>[2x]GPNCAPGQKVKLFRASEPILSVLMWGVNHTINELSNVPVPVMLMPDD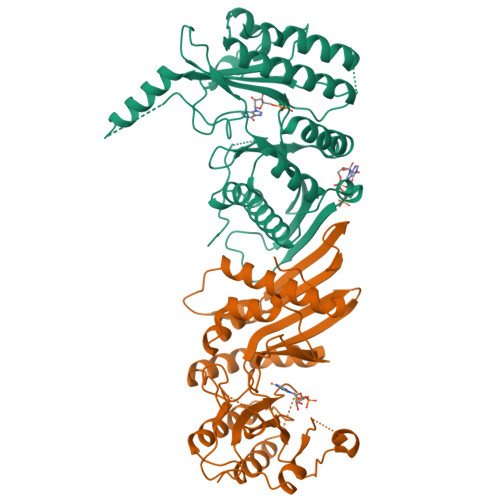FKAYSKIKVDNHLFNKENLPSRFKFKEYCPMVFRNLRERFGIDDQDYQNSVTRSAPINSDSQGRCGTRFLTTYDRRFVIKTVSSEDVAEMHNILKKYHQFIVECHGNTLLPQFLGMYRLTVDGVETYMVVTRDVFSHRLTVHRKYDLKGSTVAREASDKEKAKDLPTFKDNDFLNEGQKLHVGEESKKNFLEKLKRDVEFLAQLKIMDYSLLVGIHDVDRAEQEEMEVEERAEDEECENDGVGGNLLCSYGTPPDSPGNLLSFPRFFGPGEFDPSVDVYAMKSHESSPKKEVYFMAIIDILTPYDTKKKAAHAAKTVKHGAGAEISTVNPEQYSKRFNEFMSNILT>[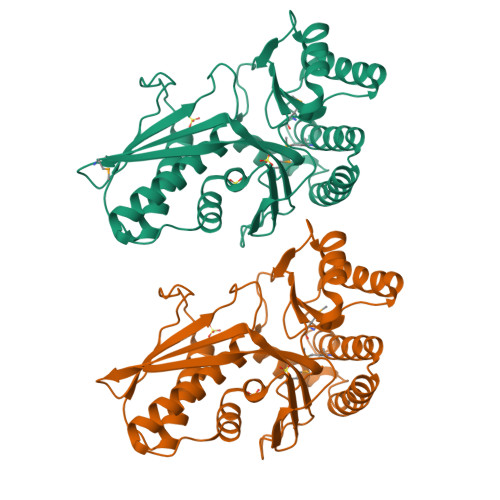2x]MHWFAQAPANIALIKYMGKKDENSNLPDNSSLSYTLSNLLSSVKLEKLPTKKDIWEPLTIPGAPEFNLSVEAQKRFIDHLVRLKEYFGYVGGFLIQSSNNFPHSSGLASSASSFAALTKCASIALSELTQKPLPSIDEQAQLSRLGSGSSCRSFYAPWALWTGDKVSAIDLPYKDLLHQVIVISSQEKEIPSRVAHKLVKTSPFYETRSERAEANLKLLLNAFENKDWTSIYQICWHEFLDMHQLFKTCEKPFSYITDNTLHILSVIEKFWNEKGDGPVVTMDAGPNVHLLYRSDQTDLARQFKSDHLVGNYDVLEGHHHHHH>[2x]MQALRRGAAIPSRLLPRRDSWMSLAPFVAPNNAAAWRKLRDGAQEVQTVIERQSTPGKPQQIDWAKWESQIAHKDILNCLKTFYTNQVQILDRALGALETAKTPAPCEGAEKGWALFDAALSACAKSVEKSEELLSNGARALWVSCSNPPVWKVNTNEWLDSDQYWQAFVEKHHFYSQYQPGVVDPEAPQEVEAFKQAWHSRMGKFNDRSDTPMLYAYMNELPSWEYYDLHRSAFLEHMTYFLVRTGGDFRFFPEMPPWQWLAHMENLRFKLLSVAQSRRSQLQLANLERERALDFLPVDVEHHGEEYTQKFLQYETELFQACAARLMGHFMFLCDPFIPVQSAEALSAVTRVDNGKGKLFSLGDDVNALFYLPEQQRRDVERPTQAVQTLLGHLEATGRPFNPCYSELLHVHAEVLEERGEHWLTAPGECVSQAFLRRLRTDDPAYEVYCSYFKEMYERFAGAKEVSMEDGRKRLATIEKNAQEEAAAYGLALKTMGSAELAHKAREGAAKLEQLRKAQEKAAGKSAQTVQENKM;>[2x]MNFSSSARWLAVRQSQTLGHTTRATVAAGRRVLAHSPAATEFTSFQSLHIGGDVCKLPLAVALGAAPSALGYGSAKHNQQRQYATLGSGWSFSKVQYTKYRITKPWTTDTTFDDIILSQPSKEDFAKFTKEAPLFLRFLKLVTDVEGRQEAFIQFAKRCENGLTVEKDVYVTKKELVDCLWKNGYTDTEINAFEIAFPADYKFHYPELAVLFDLTEEDCYKYCIRQRAATPEELVELKYTKPKNLVSSYGLCFLGVWFGLSNTVLSNAWFYSKTFPFGAVFYMLGSYFYRDIREKLWKEEKSLIHTAQENKNMGEESVYKQMKKYATDTKCLDYLSTFRTEVEDQIANYKVALVSQMRRQLTERLVEKLNGIQQAEKLIQGSLQDVMIREIVSSFKDLYKSRPELHDAAMQSAIQGLSGSDGAMDPVGAHFKASLQELAKVNLSTATADPMGTVVQRVAAVFQKREKEFLDTFTVKATEAQEIKTIVDKCHKGNTFDFHALSDEELRRLEQLYSTVNNRVGFETIHENSIKPVAPLSENSKGFVEFVNTQLEITKAKLRNARLTAFAHAFV;>MGGGGGGALNKLFPGYKDKIWMKVPVQWRQQMIQHWNKSYEKQVYSESVALNRTFQARNQLVLDRLKPSGAYRLPAVDYKRQLSRGTLVEGADFYLPTAQEQQRLARHFEPYSEQEQEERRKFRFQSISVYLAVALGASFVHDYFYQRRPVAWCLEKEPPHPPSYPFWFKSLFHSHDIPSVRRGYEVYRKVCATCHSMEQLHFRHLVGEVLPEKRVKQIAAEYDVTDGPNDQGEMYTRPGILGDAFPSPYPNEEAARYANGGAYPPDLSLITAARHFGPDYLMALLGGYRDPPEGVELRPGLYWNVWFPGNAIAMPPPLMDEMIDYEDGTPCNISQMSKDVVNFLTWATEPTADERKLYGLKCVSAIAIGTVLMTLWWRFYWAMYATRRIDFGKLKYL[2x];>MSPVGRLFLGSKLPAQTWQSFRLQPALPQFAQKRFFSGGAAKPSWHVAREHRFGPTLPDHAYYGEHATYNYFVLFIRGMRPYLEKIFGDCASTIKNAAVAVYRPVNAFVVKHNPDLRLQFVAFASFIATHMAITKEFNDMYQRLVDITSLLELQAAQLHASEGFWDSESEQQEARLQRHAEHRNDLETTWEEALREATLARNFDVLVSYLNHGTSDGCGEHGACGHSGQNGIPPSVTWNFNAMPYGKENPDTKTFPIPDHEQPYRAFSLGFTANNLSGNWGDYIDRQDNKNALMRPARMMFTDVFIPTTK[2x];>[2x]MGEKQEEEGEEEKEGKGEGGGEGGREEEDEDGSAPVVSWLRIVEERECHEETDEAPETKIALPFSAQRSSRGFEARQVEVLVSANSAFLLSVLLASLFLSSSLPSFCPPRFLLSVLLALFKDKMAGDAPAAAAAPQQAGRTASASGVRTPGYLDLVGHSLKATSMDHGMQYSSIYWETSHRTYLPFWASLTQKFSWKIMDDQIRSFLRLPKPVTTEPFVFSSGSPYIRRYFGDADISVPVPLHAPAHFAFVPTGTVSPWEETGMETGPQGAAARGAAATAFRAVLESAWKCDIDEQIKEKLHSRAGAGAFHASGSTGGCPIPTDF;>MALNRVPSRVLPFAVSGVYVHPRNACRLPAAAAVSSVPSSVSAFSSRTNFLSRSSSAVMSHPCAATARHFSFAIPPANAAALADPLPATPTPPPVFEAVSSASSGIASGTNALKNVEEVSTMERYEAAVYEESFKKPIVCLFFARFSLQSKVLLQPFLDFAASASNNATFFLIDCDRVPRAAYHARVENVPSLVVMKGDDAFRQTITDSVGVKTAGDLIQEARSALDQVLRLDQQEGGTKLQPGVSSYTHHIGVDNLNVYRKGWPVA[2x];>MQNGVFTRENADFLVKSGADSPSSQSLLLRTSPSPLSLPRRRFIFLRSASVDLSERSSLACLAPFFCLASGVCLRSAFSLPFFARRGRPCLFFIFIFFFRVSFTANFRGKRVKMAASTIPISQWPSLLYAPPSSPANPAVEALPEMQFDDLHYPRQMLLCRGAGYSLEQCNRMAQPDARVTPENPAEKLLKEEAVAAIACLSQREGGKDEQCRYYIERMYKLANKEKQPEPGTLSKASTLACKLLGIHRPEA[2x];>[2x]MAETREGGQSGAASILGAEAFPELLSKVPLNPQMDEDKHFNKYKWGNEPIPVNRRTGSRMNSSIYDNRNHEAVRHPWSTDARTFHPNDNPEADRINTQYSNMVSDSFPEGGFSDAPRFSSNWERLLAYHHGLYSPEKFNSTTKTADEIRLAVNDFAAKVHADDPKNACKYLMIEEFKCLQSAQARIDPQGAATKCVKWFNEWRQCAWDQEKMVKGYNYIEDRRARKHKPYIGAPDLQYS;>[2x]MPSSSSEDAQGGNRFECVSNSTSPRRKNATKDEAACLQPRRSAVSGPREDVLCIRTTPQPHVRRGKSGPGRRKRMRFGRERERRDKKRGEGERKRTRFPFLRLHIEGGNANSRRPLCFPSRHSLLRNHYGSLSMAFRKVSPPKAPMSVFEARSSFLDLEQCARAAGPQRWEAECQGVRQRALQAAADVMSRECGAYGDSFFQCYRHGFRLEACQGEKATMQLLRCQRMVADRLVPL;>[2x]MGLSPAFAATAGCRLASPVANSSRFLSLLRLSRPRLNAAAPAAEAAKTLERNVPMKEILQPLWVVEPPNFLRQPVWKQFWEAQFANRSFFFFGNAWTSAAAFAFFIWWSRVFDPPPKERLDRYWLNSPKFRILSAFHNPGKRPGLKISLMTYEARYCYRGLDHPFTLNEMKDFLFKLREQYLVNKYEGIQFPFVFRQFNRVSTPGTLEVHTSPALQQQPHFHEEAAGHH;>MAAGSRFPFCTAARLSSRGTLPRLGEATFFAGAESQRSAGAFAKTLQRPFLRAPSTQLFPVGNRLGVSSARALVANAMEPRRFFAAAASAKATHALQPTGTGSVAFTRPGQGSNAQFQTSLADKTRGLLGVGFLRPTKMASFAATFLLNFRFYFMYMARTTFQAVRPLLAFSVFGEVMKLVLATMSSGLFSFLFSFVLAFEVFYFFLQCYISYTFLTMFFTVLF[2x];>[2x]MTALPPPPSANVAVSFTAAPAEPLSRGEVKAASLKLELQNIERELKDWWMSRKILRDRNIGLFNLLQHHNFAGLSVNNAKLSDSQRVMWTDLVQGKPDVEDKLSVDAREMKVDMYEKLFKQAADLENPCRMPGVAYLRCLRDTLTETQSARRSSCLNAFSSFDACRTGLLKQQSAAVENSLVRQNMADVRAKALFERRAVLLDLVEGK;>[2x]MNTFFLTPAAAAARRVAVSFFARSSASGFPQHRVALRPFPSQRPAERAHNLAKSQTLRSVKAHGRQSGKKEQSTESGGRRGFRAAVGAGTGCMLAASPMLFTDYDNTASPKSELIFMAGNALGYCTERFFENEYGQSIFMFALGLAYLAMLGHEGKIHGAVWRMKHLFATNFKMVGHPRYAYALPKNPLLQDAAPTKTGSTSAKK;>[2x]MSGDSVAPHQRAACEQLHSEYKQCLAKNGRTHFSACTDFHSKLRACENMLGTSYCIDEGINLMKCTKNPDPSFCAKEFVAMRECNRPQGPHLVLSSSPSSPPHYELRPEVKHLYNVDSTDLGSAVAPVRSKEQLDRVADSLKADLNLPGYGHIPYKWESLRPNPGA;>MAFAGAAAPLGVKGRSVFAGMRSFIGQRLGRLYDSFYYSQSSTKYVMVFLFPAGIFYTRFRADTKLGYHVFINEEKLYPDYSQNYFDTKWTNGRKVYLDDETTVEQLKAQIYGGKAAPENVKVACRGRVFEDADNVAMAVRAFCKRDPRLLLFQDNL[2x];>MSPPTASASVASSGSSPHMDRLLGDLKLLAAYDSAAGWQEPKAMESAFQSLSWDDADVLKALPQYLNCRGEQKRRVDFAYAALCPRPVDEKDPKQTLMSLWMKARLFSYDQKHPFVLSPFAATDKSTSAGAMTAEKPF[2x];>MVRNQRYPASPVQEIFLPEPVPFVQFDQTAPSPNSPPAPLPSPSLSQCEEQKDRYRDISSMFHRGVAGAEQVREAYNSMAKCFRRVSVAEVLESDPAFRQARNFTMDLKQAEDDQRYKQLQYGRVPSILTKYHL[2x];>[2x]MLNFIPKRCPSVSLLFGKRPVQRIEVGQARHQLEIPVETIEKIYEGVDSRLEYHNKDYNAMKWKDFMKLKLDAYHLLEASQSETAAKSALSDLNWFSDLADIYSGQQTMAEMDVALKAQGEQKLSYPIQGKNIK;>[2x]MSWATRLLRMSSPRLGLLPLGRSVKLGGAKERVSFSQFFDSEYFWTKANVGPFFLFLFTSPFWYQGIKTVYASCRYRKLNEREIISDRYTWLHERMLEDEVERVLLEQVPAGGFDKTRPGLLLGPSTL;>MPAPAASGAAAVLSKDIARSFRWMQAFAAVKGKPTAGSCAAGTAVVNPEDPTKVTLKGRYTNFSLQHIWEKYDYLQTHLLLRECMLSQVAKNPRLLDPEINAGLTPTVFMRVPPETQDPETQAKAAPQKGQAN[2x];>MATPPLQDGAPTNGGAATKPSCGARLQNFARMAIKGPSVPHSILFGVGAGCCAYAGYYLYRAMRLTFFDTESVALQSRLRYAEKQKLFHQELDRELAAGHIASLVAEYDPVATRLPFQPMQDRYRV[2x];>[2x]MGFHFQQYIAMAGRAINPVQWTRAWRRMEGKSATEVYRDALAWTNNQFAQISRASQYRAWWWQNPLGMGLVLYGTYKAWHMIYMVRKQKKTAQLVAAAYGQGGQWLNPVPR;>MPFMWRQRAYCAPVPSAFASQQPNGLGGEAGVRKPLLRSNSESLSVFSQIPDGLLGHTTSVTMGNSDIFFLPKPSNLLKIALPAFVFMPNLTIFTRAFPFYAHTSA[2x];>MSTSPGLAFANLTLLLDVPQLPAIWAVNAWRELNGLFTEMKTLAGTSDLLYPSNRYNPQNEKTNRMGRPRKYNHGEWMFGNSY[2x]

F-type ATP synthases are energy-converting membrane protein complexes that synthesize adenosine triphosphate (ATP) from ADP and inorganic phosphate. These universal enzymes function by using the energy stored in an electrochemical potential across the bioenergetic membrane by rotary catalysis. In mitochondria, F1Fo ATP synthase resides in the crista membrane where it is known to form dimers, which can further assemble into rows critical for inducing the membrane curvature and maintaining membrane potential and morphology. Here, we investigate the mechanism for the generation of the unique cristae in the Apicomplexa, using a combination of single-particle cryo-EM, cryo-ET and subtomogram averaging.

The enlarged T. gondii Fo subcomplex differs markedly in its overall architecture from other ATP synthase structures. It displays distinct structural features including a peripheral matrix-exposed part that we term ‘wing’ region and a 360-kDa lumenal region. The Fo periphery contains several compact folds, including three coiled-coil-helix-coiled-coil-helix domain (CHCHD) containing proteins ATPTG7-9; a thioredoxin-like fold in ATPTG4; and ubiquitin-like fold in subunit-k. The dimerization interface in the membrane and lumenal regions is governed by homotypic interactions between symmetry-related subunits, most of which extend deep into both monomers. Subunit-b contains two transmembrane helices, each binds one of the symmetry-related subunit-a copies, which are therefore linked by four transmembrane helices. In addition, two cardiolipins are found on the matrix side, forming specific protein-lipid interactions bridging the two copies of subunit-b and subunit-f. This cardiolipin pair is sequestered in the Fo subcomplex with no apparent path to the bulk membrane, suggesting a structural role. An additional 15 cardiolipins and 12 other phospholipids were found to mediate a network of interactions throughout the membrane region. We traced two cavities in the Fo subcomplex corresponding to the proton half-channels on the lumenal and matrix sides. Taken together, both half-channels are partially lined by apicomplexan-specific subunits resulting in a divergent structure and likely the involvement of different residues in proton translocation compared to structures from other organisms.> NREEKILNREIGFAIGMPVCEFDMVKDPEVQDFRRNILNVCKEAVDLRDLNSPHSRAMYVYPPNVESSPELPKHIYNKLDKGQIIVVIWVIVSPNNDKQKYTLKINHDCVPEQVIAEAIRKKTRSMLLSSEQLKLCVLEYQGKYILKVCGCDEYFLEKYPLSQYKYIRSCIMLGRMPNLMLMAKESLYSQLPMDCFTMPSYSRRISTATPYMNGETSTKSLWVINSALRIKILCATYVNVNIRDIDKIYVRTGIYHGGEPLCDNVNTQRVPCSNPRWNEWLNYDIYIPDLPRAARLCLSICSVKGRKGAKEEHCPLAWGNINLFDYTDTLVSGKMALNLWPVPHGLEDLLNPIGVTGSNPNKETPCLELEFDWFSSVVKFPDMSVIEEHANWSVSREAGFSYSHAGLSNRLARDNELRENDKEQLKAISTRDPLSEITEQEKDFLWSHRHYCVTIPEILPKLLLSVKWNSRDEVAQMYCLVKDWPPIKPEQAMELLDCNYPDPMVRGFAVRCLEKYLTDDKLSQYLIQLVQVLKYEQYLDNLLVRFLLKKALTNQRIGHFFFWHLKSEMHNKTVSQRFGLLLESYCRACGMYLKHLNRQVEAMEKLINLTDILKQEKKDETQKVQMKFLVEQMRRPDFMDALQGFLSPLNPAHQLGNLRLEECRIMSSAKRPLWLNWENPDIMSELLFQNNEIIFKNGDDLRQDMLTLQIIRIMENIWQNQGLDLRMLPYGCLSIGDCVGLIEVVRNSHTIMQIQCKGGLKGALQFNSHTLHQWLKDKNKGEIYDAAIDLFTRSCAGYCVATFILGIGDRHNSNIMVKDDGQLFHIDFGHFLDHKKKKFGYKRERVPFVLTQDFLIVISKGAQECTKTREFERFQEMCYKAYLAIRQHANLFINLFSMMLGS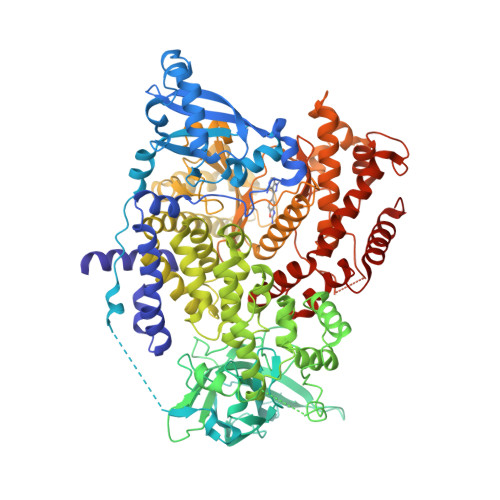GMPELQSFDDIAYIRKTLALDKTEQEALEYFMKQMNDAHHGGW>[8x]SNAMNEMTHRTKTRPVK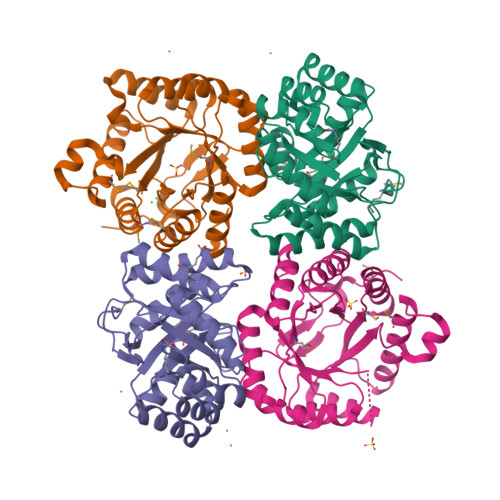VGNLTIGGNNELIIQSMTTTKTHDVEATVAEIKRLEEAGCQVVRVAVPDERAANAIADIKKQINIPLVADIHFDYRLALKAIEGGIDKVRINPGNIGRRHKVEAVVNAAKERGIPIRIGVNAGSLERHILEKYGYPTADGMVESALHHIKILEDLDFHDIIVSMKASDVNLAIEAYEKAARAFDYPLHLGITESGTLFAGTVKSAAGLGAILNKGIGNTLRISLSADPVEEVKVARELLKSFGLASNAATLISCPTCGR> NTLDTLYKEQIAEDIVWDIIDELE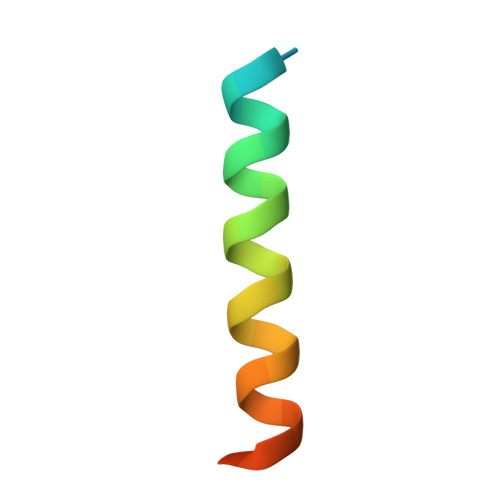QIALQQ> GPGYQDPMNIIEQKFYDSKAFFNTQQTKDISFRKEQLKKLSKAIKSYESDILEALYTDLGKNKVEAYATEIGITLKSIKIARKELKNWTKTKNVDTPLYLFPTKSYIKKEPYGTVLIIAPFNYPFQLVFEPLIGAIAAGNTAIIKPSELTPNVARVIKRLINETFDANYIEVIEGGIEETQTLIHLPFDYVFFTGSENVGKIVYQAASENLVPVTLEMGGKSPVIVDETANIKVASERICFGKFTNAGQTSVAPDYILVHESVKDDLITALSKTLREFYGQN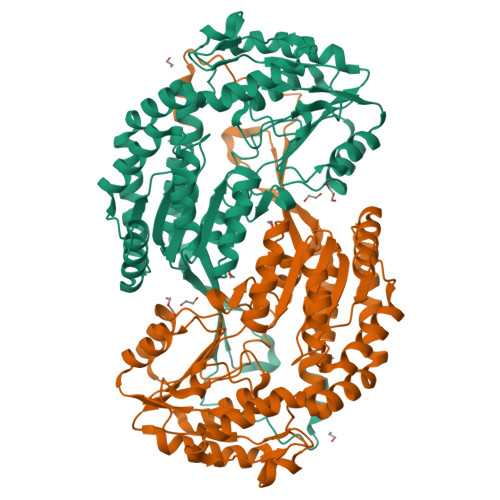IQQSPDYGRIVNLKHYHRLTSLLNSAQMNIVFGGHSDEDERYIEPTLLDHVTSDSAIMQEEIFGPILPILTYQSLDEAIAFIHQRPKPLSLYLFSEDENATQRVINELSFGGGAINDTLMHLANPKLPFGGVGASGMGRYHGKYSFDTFTHEKSYIFKSTRLESGVHLPPYKGKFKYIKAFFKN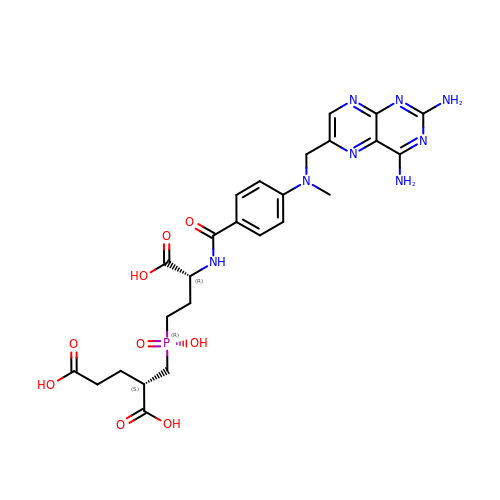(2S)-2-{[(R)-[(3R)-3-carboxy-3-{[(4-{[(2,4-diaminopteridin-6-yl)methyl](methyl)amino}phenyl)carbonyl]amino}propyl](hydroxy)phosphoryl]methyl}pentanedioic acid | C25 H31 N8 O9 P | BHCAHIKEPKIXJL-RHSMWYFYSA-N ethyl 4-chloranyl-1-methyl-6-oxidanylidene-pyridine-3-carboxylate | C9 H10 Cl N O3 | 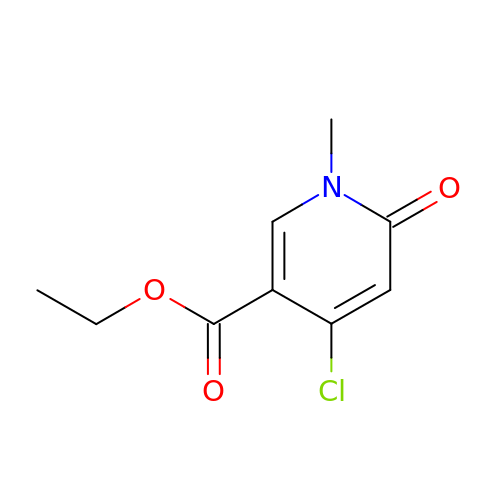WGSWOEOJYNQPRP-UHFFFAOYSA-N Clathrin mediates vesicular transport between post‐Golgi membranes in eukaryotes and is targeted to specific membranes by interactions with clathrin adaptor proteins. A total of 3 consensus clathrin‐binding peptide sequences have been identified and structural studies show that each binds distinct sites on the clathrin heavy chain N‐terminal domain (NTD). We have solved high‐resolution structures of NTD bound to peptide motifs from the cellular clathrin adaptors β2 adaptin and amphiphysin plus a putative viral clathrin adaptor, hepatitis D virus large antigen (HDAg‐L). Surprisingly, with each peptide we observe simultaneous peptide binding at multiple sites on NTD and viral peptides binding to the same sites as cellular peptides.

In all the structures presented a peptide could be observed at the “clathrin box”, lying between blades 1 and 2 of the NTD β‐propeller fold (“clathrin box”). For the cellular peptides (AP2CBMpep, AmphCBMpep and Amph4T1pep) the binding is similar to that previously described, with the 3 leucine side chains of the CBM LΦxΦ[DE] consensus sequence occupying the hydrophobic pocket formed at the groove between the 2 blades. In addition to binding at the clathrin box, we observed significant binding of the cellular peptides (AP2CBMpep, AmphCBMpep and Amph4T1pep) at the “arrestin box”, which lies between blades 4 and 5 of the NTD β‐propeller fold (“arrestin box”). While all 3 CBM peptides bind in the same general orientation at the arrestin box, the molecular details of these interactions differ from the interaction seen between NTD and the extended surface loop of the arrestin 2 long isoform (arrestin2L). Most notably, the directionality of the peptide chain is reversed. The first 2 leucine residues of each CBM (LΦxΦ[DE]) bind in a hydrophobic cavity lined by the side chains of NTD residues W164, L183, S185, R188, V190, I194, F216, I231 and V233 plus the peptide backbones of Y184 and S191. His‐NTD‐NEMO with mutations at the clathrin box was less efficiently captured by GST‐AP2CBM, the defect being most pronounced for the Q89A + F91K mutant, but capture of these mutants by GST‐AmphCBM or GST‐Amph4T1 was largely unperturbed. Similarly, His‐NTD‐NEMO mutated at the arrestin box (Q192Y) was captured less efficiently by GST‐AP2CBM but the capture of this mutant by GST‐AmphCBM or GST‐Amph4T1 was not significantly changed. While His‐NTD‐NEMO mutated at either the clathrin box (Q89A + F91K) or arrestin box (Q192Y) can still be captured by GST‐AP2CBM, combining the mutations (Q89A + F91K + Q192Y) reduces the binding to the level of the GST control. We observe that combining mutations at the arrestin and clathrin boxes completely abolishes the ability of the AP2CBM to capture NTD in GST pull‐down assays, confirming that CBM peptides bind promiscuously to both sites.

> GSMAQILPIRFQEHLQLQNLGINPANIGFSTLTMESDKFICIREKVGEQAQVVIIDMNDPSNPIRRPISADSAIMNPASKVIALKAGKTLQIFNIEMKSKMKAHTMTDDVTFWKWISLNTVALVTDNAVYHWSMEGESQPVKMFDRHSSLAGCQIINYRTDAKQKWLLLTGISAQQNRVVGAMQLYSVDRKVSQPIEGHAASFAQFKMEGNAEESTLFCFAVRGQAGGKLHIIEVGTPPTGNQPFPKKAVDVFFPPEAQNDFPVAMQISEKHDVVFLITKYGYIHLYDLETGTCIYMNRISGETIFVTAPHEATAGIIGVNRKGQVLSVCVEEENIIPYITNVLQNPDLALRMAVRNNLAGAEEL;>[2x]CGDLLNLDLG>[2x]KETAAAKFERQHMDSSTSAASSSNYCNQMMKSRNLTKDRCKPVNTFVHESLADVQAVCSQKNVACKNGQTNCYQSYSTMSITDCRETGSSKYPNCAYKTTQANKHIIVACEGNPYVPVHFDASV

With the new chain-extended nucleoside oligophosphates in hand, we go on to investigate in detail their interaction with ribonuclease A, a model protein containing a polycationic active site and for which X-ray crystal structures are relatively straightforward to obtain. Thus, we go on to investigate in detail the interaction of the polyanionic constructs with ribonuclease A, a model protein containing a polycationic active site and for which X-ray crystal structures are relatively straightforward to obtain. This work presents a combined experimental and quantum chemical approach to understanding the interactions of RNase A with the new nucleoside hexa- and heptaphosphate constructs. To better comprehend RNase A and nucleoside oligophosphate interactions, we examine the correlation between the experimental and calculated protein–ligand interactions by combining efforts in crystallographic and computational investigations in the present work. The combination of the CCSD(T) approach with the appropriate energy decomposition scheme enables deciphering the influence of the oligophosphate chain length and of individual polypeptide and nucleoside residues on ligand binding.

Here, we demonstrate by extending adenosine monophosphate (AMP) and uridine monophosphate (UMP) to their corresponding nucleoside hexaphosphates, while adenosine diphosphate (ADP) and uridine diphosphate (UDP) are phosphate chain-extended to the corresponding nucleoside heptaphosphates. In the presence of Mo(NCMe)3(CO)3,35 [PPN]2[TBA]1 readily reacted with anhydrous NMPs and NDPs, yielding the corresponding hexa- and heptaphosphates after subsequent hydrolysis. Anion-exchange HPLC purification of the resulting compounds provided the ammonium salts of adenosine/uridine hexaphosphates (50% yield for p6A and 29% for p6U) and adenosine/uridine heptaphosphates (24% yield for p7A and 17% for p7U). This result represents the first direct chemical syntheses of nucleoside-5′-hexa- and -heptaphosphates. Additionally, we found that the hydrolytic ring-opening process exhibits less selectivity when leading to the nucleoside heptaphosphates as compared with that leading to the nucleoside hexaphosphates, with observed formation of pentametaphosphate and NDPs. Aqueous solutions of the purified nucleoside hexa- and heptaphosphates were observed to be stable for at least a week, as confirmed by 31P{1H} NMR spectroscopy.> MSGPERITLAMTGASGAQYGLRLLDCLVQEEREVHFLISKAAQLVMATETDVALPAKPQAMQAFLTEYCGAAAGQIRVFGQNDWMAPPASGSSAPNAMVICPCSTGTLSAVATGACNNLIERAADVALKERRPLVLVPREAPFSSIHLENM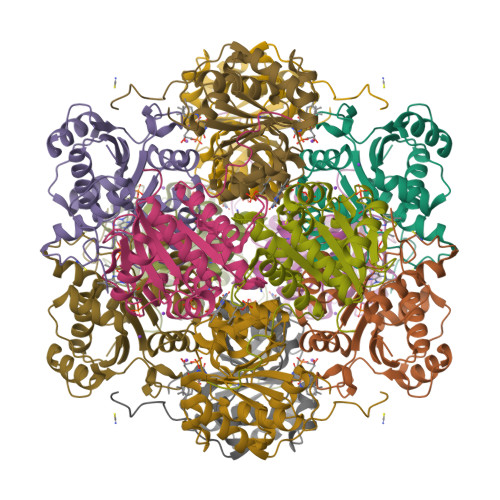LKLSNLGAVILPAAPGFFHQPQSVEDLVDFVVARILNTLGIPQDMLPRWGEQHLVSDE>[3x]MAADAPAASQQSKPSESDKSESSMSSHAPVVFTLRTGIAEGRMVYIGVGGDIDRQVNPKLVVHEGETVQINLINGEGAQHDAVIDQYAARSAIVSGKNASSTFSFIASKVGQFDYYCSLPGHRQAGMQGVLQVVPGNRAEMPSTAADITRDPADLPGPIGARQAKTVRIDLETVELKGQLDDKTTYTYWTFNGKVPGPFLRVRVGDTVELHLKNAKDSLMIHSVDFHGATGPGGAAAYTQTDPGAETVVTFKALVPGIFVYHCATPSVPNHITNGMYGLLLVEPEGGLPQVDREFYVMQGEIYTVKPFGTSGEQEMDYEKLISEKPEYFLFNGSVGALTRTHPLYANVGETVRIFFGVGGPNFTSSFHVIGEIFDHVYALGSVTSPPLTGVQTVSVPPGGATIVDFKLDRGGRYVLVDHALSRLDHGLVGFLNVDGPKNDAIMHEGPPKQENLYFQ

Copper-containing nitrite reductases (CuNiRs) are found in all three kingdoms of life and play a major role in the denitrification branch of the global nitro­gen cycle where nitrate is used in place of di­oxy­gen as an electron acceptor in respiratory energy metabolism. The catalytic type-2 copper center (T2Cu) is located at the interface of the adjacent monomers and is ‘hard-wired’ to the electron-donating type-1 copper center (T1Cu) via neighboring residues that form a Cys–His electron-transfer (ET) bridge. The two active-site residues, AspCAT and HisCAT around the T2Cu, are involved in substrate binding and catalysis with both residues starting in the deprotonated state prior to substrate-binding events. The hexameric structure observed for the N-terminal cupredoxin-tethered three-domain CuNiR from two strains of Hyphomicrobium denitrificans suggests that it is likely to offer an advantage for these organisms.

Intriguingly, three T2Cu sites belonging to the trimer in the asymmetric unit are occupied by different ligands: two by the substrate nitrite and one by a diatomic molecule consistent with it being the product nitric oxide. Each of these independent sites have full occupancy of copper and the ligand. The product may have formed from enzyme turnover catalyzed by solvated electrons generated during X-ray data collection, but the full occupancy of a single species is surprising. This suggests a very slow off-rate for dissociation of the product which is consistent with the lower NiR activity in these enzymes. In this case both the water and His27 itself show poorer electron density compared with the other two structures, suggesting higher flexibility of the N-terminal peptide that may facilitate release of the NO from the T2Cu with consequent return to the resting state. The conformational flexibility of this N-terminal peptide and His27 may be critical for the substrate entry, anchoring and product formation stages of the catalytic reaction, requiring it to move to the outward conformation for the eventual release of the product. The observation of side-on NO binding geometry seen here adds to the gathering evidence that this geometry is energetically stable at the T2Cu site of CuNiR and is an intrinsic part of the catalytic turnover.> MTDTTNSIKH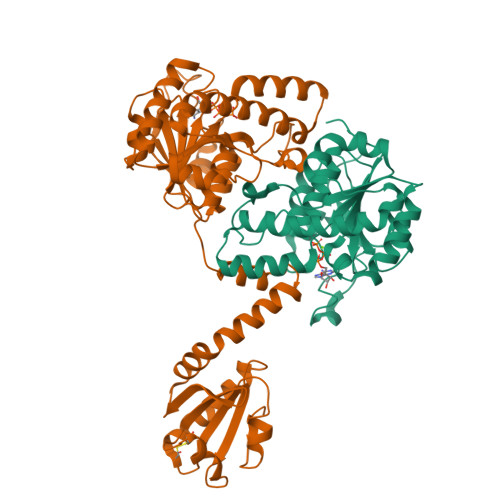VISPLARQTLQDRDLTRPVAGKRPIRLLPWLQVVKIGGRVMDRGADAILPLVEELRKLLPEHRLLILTGAGVRARHVFSVGLDLGLPVGSLAPLAASEAGQNGHILAAMLASEGVSYVEHPTVADQLAIHLSATRAVVGSAFPPYHHHEFPGSRIPPHRADTGAFLLADAFGAAGLTIVENVDGIYTADPNGPDRGQARFLPETSATDLAKSEGPLPVDRALLDVMATARHIERVQVVNGLVPGRLTAALRGEHVGTLIRTGVRPAENLYFQGSAWSHPQFEK;> MGSDKIIHLTDDSFDTDVLKADGAILVDFWAEWCGPCKMIAPILDEIADEYQGKLTVAKLNIDQNPGTAPKYGIRGIPTLLLFKNGEVAATKVGALSKGQLKEFLDANLEEEKRKREEELLMQRSLTDPQLQAAAAAAADFRILPDATVIKIGGQSVIDRGRAAVYPLVDEIVAARKNHKLLIGTGAGTRARHLYSIAAGLGLPAGVLAQLGSSVADQNAAMLGQLLAKHGIPVVGGAGLSAVPLSLAEVNAVVFSGMPPYKLWMRPAAEGVIPPYRTDAGCFLLAEQFGCKQMIFVKDEDGLYTANPKTSKDATFIPRISVDEMKAKGLHDSILEFPVLDLLQSAQHVREVQVVNGLVPGNLTRALAGEHVGTIITAS Pyrrolidine | C4 H9 N | 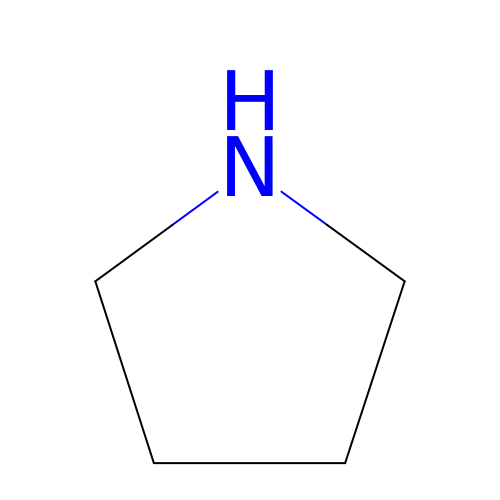RWRDLPDLKQPQOW-UHFFFAOYSA-N>NSGMLEEDLIQYYQFLAEKGDVQAQVGLGQLHLHGGRGVEQNHQRAFDYFNLAANAGNSHAMAFLGKMYSEGSDIVPQSNETALHYFKKAADMGNPVGQSGLGMAYLYGRGVQVNYDLALKYFQKAAEQGWVDGQLQLGSM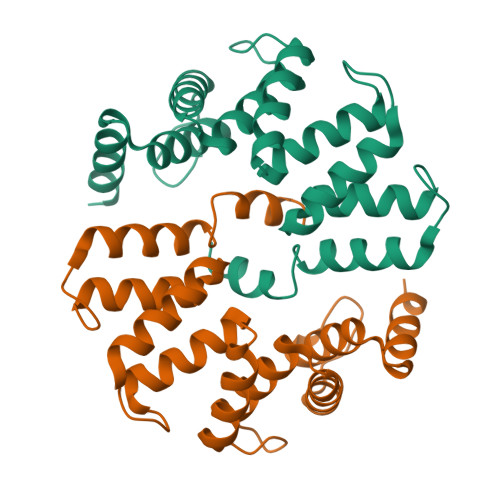YYNGIGVKRDYKQALKYFNLASQGGHILAFYNLAQMHASGTGVMR[4x]>[4x]MATQGVFTLPANTRFGVTAFANSSGTQTVNVLVNNETAATFSGQSTNNAVIGTQVLNSGSSGKVQVQVSVNGRPSDLVSAQVILTNELNFALVGSEDGTDNDYNDAVVVINWPLG;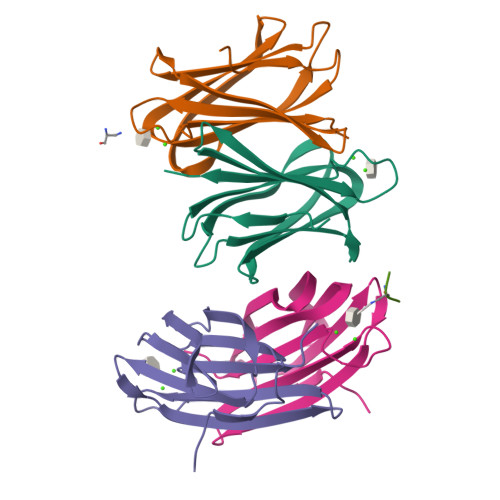>KAY[2x]> MEDVEIKPRGYQLRLVDHLTKSNGIVYLPTGSGKTFVAILVLKRFSQDFDKPIESGGKRALFMCNTVELARQQAMAVRRCTNFKVGFYVGEQGVDDWTRGMWSDEIKKN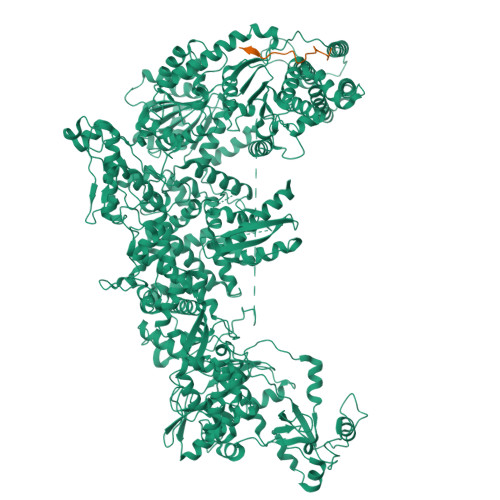QVLVGTAQVFLDMVTQTYVALSSLSVVIIDECHHGTGHHPFREFMRLFTIANQTKLPRVVGLTGVLIKGNEITNVATKLKELEITYRGNIITVSDTKEMENVMLYATKPTEVMVSFPHQEQVLTVTRLISAEIEKFYVSLDLMNIGVQPIRRSKSLQCLRDPSKKSFVKQLFNDFLYQMKEYGIYAASIAIISLIVEFDIKRRQAETLSVKLMHRTALTLCEKIRHLLVQKLQDMTYDDDDDNVNTEEVIMNFSTPKVQRFLMSLKVSFADKDPKDICCLVFVERRYTCKCIYGLLLNYIQSTPELRNVLTPQFMVGRNNISPDFESVLERKWQKSAIQQFRDGNANLMICSSVLEEGIDVQACNHVFILDPVKTFNMYVQSKGRARTTEAKFVLFTADKEREKTIQQIYQYRKAHNDIAEYLKDRVLEKTEPELYEIKGHFQDDIDPFTNENGAVLLPNNALAILHRYCQTIPTDAFGFVIPWFHVLQEDERDRIFGVSAKGKHVISINMPVNCMLRDTIYSDPMDNVKTAKISAAFKACKVLYSLGELNERFVPKTLKERVASIADVHFEHWNKYGDSVTATVNKADKSKDRTYKTECPLEFYDALPRVGEICYAYEIFLEPQFESCEYTEHMYLNLQTPRNYAILLRNKLPRLAEMPLFSNQGKLHVRVANAPLEVIIQNSEQLELLHQFHGMVFRDILKIWHPFFVLDRRSKENSYLVVPLILGAGEQKCFDWELMTNFRRLPQSHGSNVQQREQQPAPRPEDFEGKIVTQWYANYDKPMLVTKVHRELTPLSYMEKNQQDKTYYEFTMSKYGNRIGDVVHKDKFMIEVRDLTEQLTFYVHNRGKFNAKSKAKMKVILIPELCFNFNFPGDLWLKLIFLPSILNRMYFLLHAEALRKRFNTYLNLHLLPFNGTDYMPRPLEIDYSLKRNVDPLGNVIPTEDIEEPKSLLEPMPTKSIEASVANLEITEFENPWQKYMEPVDLSRNLLSTYPVELDYYYHFSVGNVCEMNEMDFEDKEYWAKNQFHMPTGNIYGNRTPAKTNANVPALMPSKPTVRGKVKPLLILQKTVSKEHITPAEQGEFLAAITASSAADVFDMERLEILGNSFLKLSATLYLASKYSDWNEGTLTEVKSKLVSNRNLLFCLIDADIPKTLNTIQFTPRYTWLPPGISLPHNVLALWRENPEFAKIIGPHNLRDLALGDEESLVKGNCSDINYNRFVEGCRANGQSFYAGADFSSEVNFCVGLVTIPNKVIADTLEALLGVIVKNYGLQHAFKMLEYFKICRADIDKPLTQLLNLELGGKKMRANVNTTEIDGFLINHYYLEKNLGYTFKDRRYLLQALTHPSYPTNRITGSYQELEFIGNAILDFLISAYIFENNTKMNPGALTDLRSALVNNTTLACICVRHRLHFFILAENAKLSEIISKFVNFQESQGHRVTNYVRILLEEADVQPTPLDLDDELDMTELPHANKCISQEAEKGVPPKGEFNMSTNVDVPKALGDVLEALIAAVYLDCRDLQRTWEVIFNLFEPELQEFTRKVPINHIRQLVEHKHAKPVFSSPIVEGETVMVSCQFTCMEKTIKVYGFGSNKDQAKLSAAKHALQQLSKCDA;> MDQENFHGSSLPQQLQNLHIQPQQASPNPVQTGFAPRRHYNNLVGLGNGNAVSGSPVKGAPLGQRHVKLKKEKISAQVAQLSQPGQLQLSDVGDPALAGGSGLQGGVGLMGVILPSDEALKFVSETDANGLAMKTPVSILQELLSRRGITPGYELVQIEGAIHEPTFRFRVSFKDKDTPFTAMGAGRSKKEAKHAAARALIDKLIGAQLPESPSSSAGPSVTGLTVAGSGGDGNANATGGGDASDKTVGNPIGWLQEMCMQRRWPPPSYETETEVGLPHERLFTIACSILNYREMGKGKSKKIAKRLAAHRMWMRLQETPIDSGKISDSICGELEGEVSIIQDIDRYEQVSKDFEFIKI>ADKLPNIVILATGGTIAGSAATGTQTTGYKAGALGVDTLINAVPEV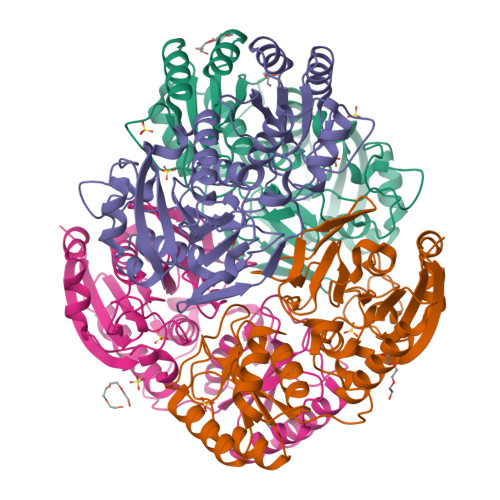KKLANVKGEQFSNMASENMTGDVVLKLSQRVNELLARDDVDGVVITHGTDTVEESAYFLHLTVKSDKPVVFVAAMRPATAISADGPMNLLEAVRVAGDKQSRGRGVMVVINDRIGSARYITKTNASTLDTFRANEEGYLGVIIGNRIYYQNRIDKLHTTRSVFDVRGLTSLPKVDILYGYQDDPEYLYDAAIQHGVKGIVYAGMGAGSVSVRGIAGMRKALEKGVVVMRSTRTGNGIVPPDEELPGLVSDSLNPAHARILLMLALTRTSDPKVIQEYFHTY[4x]> TVAAYNLTWKSTNFKTILEWEPKPVNQVYTVQISTKSGDWKSKCFYTTDTECDLTDEIVKDVKQTYLARVFSYPAGNVESTGSAGEPLYENSPEFTPYLETNLGQPTIQSFEQVGTKVNVTVEDERTLVRRNNTFLSLR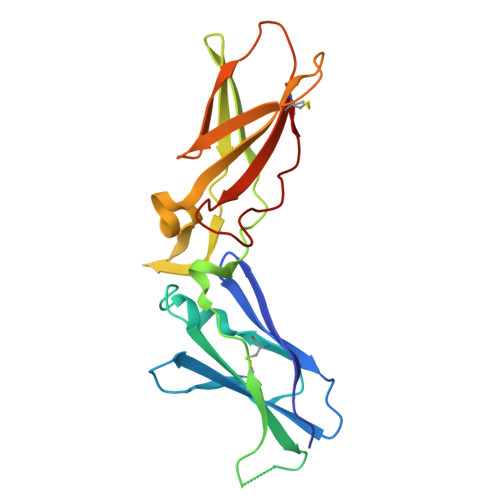DVFGKDLIYTLYYWKSSSSGKKTAKTNTNEFLIDVDKGENYCFSVQAVIPSRTVNRKSTDSPVECM8-Oxoguanine (GO) is a major purine oxidation product in DNA. The major way to remove GO is the base excision repair pathway, usually initiated by a GO-DNA glycosylase. While no enzymes with an A/G specific-DNA glycosylase or a dGOTPase activity have been discovered in these species, a GO-DNA glycosylase called AGOG (for Archaeal GO-DNA Glycosylase) has been initially identified in the hyperthermophilic archaeon Pyrobaculum aerophilum. Despite very low sequence identity, AGOG is structurally similar to eukaryotic and prokaryotic OGG1 and OGG2 GO-DNA glycosylases and, like these two proteins, belongs to the Endo III structural superfamily partly defined by the central helix-hairpin-helix (HhH) element followed by a glycine/proline-rich region and an aspartate (GPD).

To get structural insight into AGOG bound to single-stranded DNA, we crystallized rSB using Pab-AGOG and GO-containing single-stranded DNA. rSB obtained between Pab-AGOG and a 13-nucleotide single-stranded DNA containing a GO at position 7 in the presence of NaBH4 was purified to homogeneity as described in Materials and Methods. Best diffracting crystals were obtained with a 9-mer single-stranded DNA, allowing us to solve the structure of Pab-AGOG borohydride-trapped-DNA complex (Pab-AGOG_ssDNA). Four complexes were present in the crystal asymmetric unit, each showing a slightly different conformation for the DNA molecule. As expected, the covalent bond between the ϵ-amino group of K142 and the C1’ of the ring-open form of the AP site is clearly seen from the electron density confirming K142 as the catalytic nucleophile of Pab-AGOG. Few nucleotides are contacted by the enzyme: 2 and 3 nucleotides at the 5’ and 3’ side of the AP site, respectively. The single-stranded DNA is bound in the groove between the two protein domains and the HhH motif. Pab-AGOG interacts via its R93 residue with the T1 and T2 bases at the 5’ DNA extremity and via the Q53, G56, G58, Q97, R101, R104, T143 residues with the DNA phosphodiester backbone or deoxyribose of the residues PED4 (AP site) to T7. At the trapped AP site, the phosphate group fluctuates between two conformations and a large kink of about 90° is observed for the DNA backbone. In the structure, the AP site is stabilized by Oγ of S175 and the amide of the strictly conserved R176, which form hydrogen bonds with the O4’ hydroxyl group. Compared to the apo or 8-oxodG-bound structures, the protein sidechains of residues F146 and W212 show severe rearrangement concomitant with the displacement of the helices α11 and α13 of the N/C domain.

>GSHMIARIIGEIGIEGARFIEENIDEQFKALRYLSKGIDSETFVKLVIANSLVSYQLTGKGEQWWWEFAKYFYGRDVKSIYLAYKEFLPNSRFNRRLIPQKLSRIRRVETFLSTLTEERIEEYYGDMSSLWGSIARALGVDKESKTVVFSVKMFGYAARIVLSTFNPYPMEIPIPEDSRIVKLTKKLTNEKPRKFWMKIARESGVPPLHIDSILWPLLGGASIDSAPPELRDKLAELIKIIR[4x]>[5x]GQDMVSPPPPIADEPLTVNTGIYLIECYSLDDKAETFKVNAFLSLSWKDRRLAFDPVRSGVRVKTYEPEAIWIPEIRFVNVENARDADVVDISVSPDGTVQYLERFSARVLSPLDFRRYPFDSQTLHIYLIVRSVDTRNIVLAVDLEKVGKNDDVFLTGWDIESFTAVVKPANFALEDRLESKLDYQLRISRQYF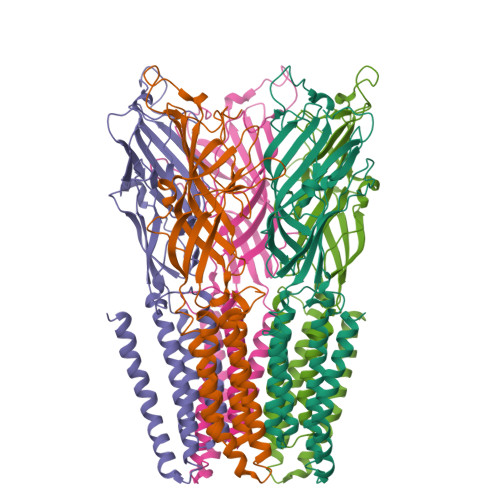SYIPNIILPMLFILFISWTAFWSTSYAANVTLVVSTLIAHIAFNILVETNLPKTPYMTYTGAIIFMIYLFYFVAVIEVTVQHYLKVESQPARAASITRASRIAFPVVFLLANIILAFLFFGF> MHHHHHHSSGRENLYFQGIPTISELKKDRIIPHVFPNDKIDLNVDLFISF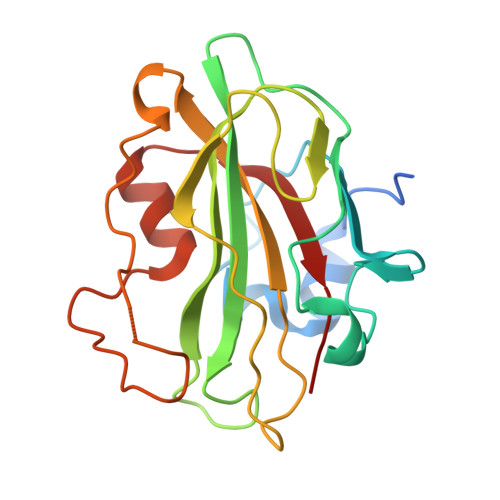KAGKEVNHGNVLDIAGTGSVPRNIKFSEEPPDGYCFVLFMVDPDYPSRLRPDGKEYIHWVVSGIKTKELIKGTQKNCVTILPYVGPSIKKGTGLHRISFIISLIKEEDKDNITGLPHYKGEKYITRVKFNNYESVHNIAQINNMKIVGYNWCQIE>[4x]KGKLPPVVHGTTPFVGHIIQFGKDPLGFMLKAKKKYGGIFTMNICGNRITVVGDVHQHSKFFTPRNEILSPREVYSFMVPVFGEGVAYAAPYPRMREQLNFLAEELTVAKFQNFAPSIQHEVRKFMKANWNKDEGEINILDDCSAMIINTACQCLFGEDLRKRLDARQFAQLLAKMESCLIPAAVFLPWILKLPLPQSYRCRDARAE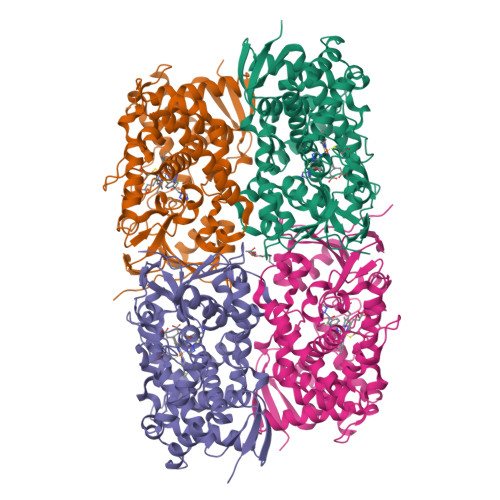LQDILSEIIIAREKEEAQKDTNTSDLLAGLLGAVYRDGTRMSQHEVCGMIVAAMFAGQHTSTITTTWSLLHLMDPRNKRHLAKLHQEIDEFPAQLNYDNVMEEMPFAEQCARESIRRDPPLVMLMRKVLKPVQVGKYVVPEGDIIACSPLLSHQDEEAFPNPREWNPERNMKLVDGAFCGFGAGVHKCIGEKFGLLQVKTVLATVLRDYDFELLGPLPEPNYHTMVVGPTASQCRVKYIKKKKAAA>MKRQGKRPSKNLKARCSRKALHVNFKDMGWDDWIIAPLEYEAFHCEGLCEFPLRSHLEPTNHAVIQTLMNSMDPESTPPTCCVPTRLSPISILFIDSANNVVYKQYEDMVVESCGCR[6x];>[18x]ETGQCRIQKCTTDFVSLTSHLNSAVDGFDSEFCKALRAYAGCTQRTSKACRGNLVYHSAVLGISDLMSQRNCSKDGPTSSTNPEVTHDPCNYHSHAGAREHRRGDQNPPSYLFCGLFGDPHLRTFKDNFQTCKVEGAWPLIDNNYLSVQVTNVPVVPGSSATATNKITIIFKAHHGCTDQKVYQAVTDDLPAAFVDGTTSGGDSDAKSLRIVERESGHYVEMHARYIGTTVFVRQVGRYLTLAIRMPEDLAMSYEESQDLQLCVNGCPLSERIDDGQGQVSAILGHSLPRTSLVQAWPGYTLETANTQCHEKMPVKDIYFQSCVFDLLTTGDANFTAAAHSALEDVEALHPRKERWHIFPSSGTKHHHHHH;>[6x]ETGTPMMPPVGVQASILSHDTIRITWADNSLPKHQKITDSRYYTVRWKTNIPANTKYKNANATTLSYLVTGLKPNTLYEFSVMVTKGRRSSTWSMTAHGA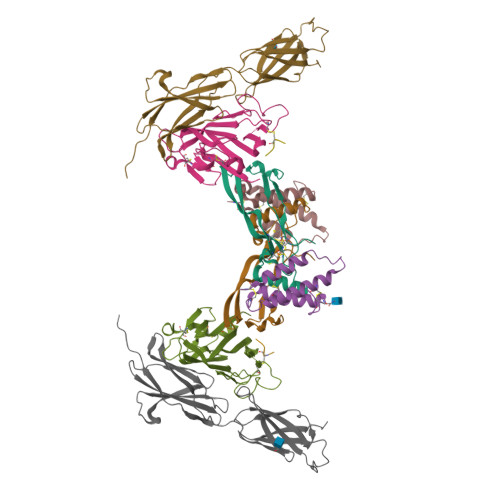TFELVPTSPPKDVTVVSKEGKPRTIIVNWQPPSEANGKITGYIIYYSTDVNAEIHDWVIEPVVGNRLTHQIQELTLDTPYYFKIQARNSKGMGPMSEAVQFRTPKALGSAGKGSRLPDLGSDYKPPMSGSNSPHGSPTSPLDSNGTKHHHHHH> RSMSRPVQEMIPLKFFAVDEVSCQINQEGAPKDVVEKVLFVLNNVTLANLNNKVDELKKS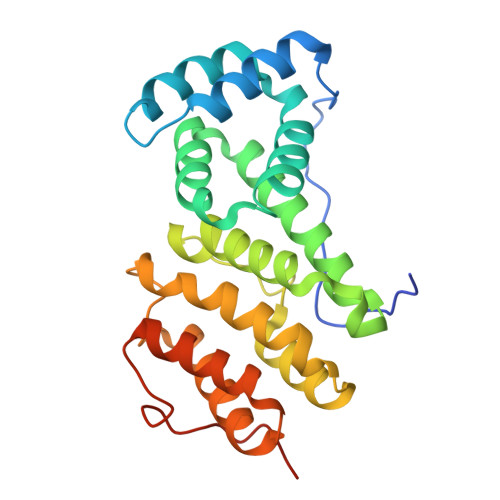LTPNYFSWFSTYLVTQRAKTEPNYHDLYSKVIVAMGSGLLHQFMVNVTLRQLFVLLSTKDEQAIDKKHLKNLASWLGCITLALNKPIKHKNIAFREMLIEAYKENRLEIVVPFVTKILQRASESKIFKPPNPWTVGILKLLIELNEKANWKLSLTFEVEVLLKSFNLTTKSLKPSNFINTPEVIETLSG>[2x]MAGRTRIPFNGVGTSVLPAYQTLSAGQYLLSPNQRFKLLLQGDGNLVIQDNGATVWVANEQQPFSSTIPLRNKKAPLAFYVQYGAFLDDYSRRRVWLTDNSTFTSNDQWNRTHLVLQDDGNIVLVDSLALWNGTPAIPLVPGAIDSLLLAPGSELVQGVVYGAGASKLVFQGDGNLVAYGPNGAATWNAGTQGKGAVRAVFQGDGNLVVYGAGNAVLWHSHTGGHASAVLRLQANGSIAILDEKPVWARFGFQPTYRHIRKINPDQKPIDIWTWHF

Putidacin A (or LlpABW), first identified in Pseudomonas putida BW11M1, represents a class of Pseudomonas-specific antibacterial proteins not related to any known bacteriocin. The crystal structure of LlpABW from P. putida BW11M1 (LlpABW) shows it contains two β-prism MMBL domains, referred to as the N-domain and the C-domain following their position in the amino acid sequence. For the protein containing two similarly folded domains, we constructed site-specific mutants affected in carbohydrate binding and domain chimers from LlpA homologues to show that mannose-specific sugar binding mediated by one domain is required for activity and that the other domain determines target strain specificity. The LlpA branch occupies a unique position among MMBL-domain proteins, harboring non-eukaryotic representatives and being equipped with the capacity to kill bacterial cells with bacteriocin-like specificity, a property not yet demonstrated for other family members.

Soaks with oligomannoses revealed additional sugar-binding subsites. Binding site IIIC accommodates the disaccharide Manα(1–2)Man and the pentasaccharide GlcNAcβ(1–2)Manα(1–3)[GlcNAcβ(1–2)Manα(1–6)]Man. In the bound disaccharide, the non-reducing mannose is located in the Man-Me binding site while the reducing mannose faces the solvent and does not interact directly with the protein. Although mannose-containing carbohydrates can bind to the IIIC pocket of LlpABW, it remains unclear if these are part of or mimic the natural ligand required for biological activity since bacteriocin activity is not impaired in the presence of excess mannose.>MEASRRDFISIGIGALGAVGGLGALYALVRVMLEPSEIAALGAKTEIDVSKIQPMQVRVTSWKGKTLFAIRLPKDFKPEGYTLKKGALNSKGTTNYEILKGHDVFALVGVCTHLGCIPLWKPQGEGGINKPVFHCPCHGGLYTPYGDVIGGPPPRPLFIPPQKLEGNKLIVGVEGFVKELI[2x];>MGLIEKIVDWIDERAHVREIYRTQMVEYKVAKNLTFPYVFGILALVTFAIQIISGMVLILYYKPSIADAFDSATYSIMGEIPFGWLFRHIHATGANFFMAIVYLHMFTGIYYNAYKRPRELVWIVGWLIYFVLILTALSGYLLPWGQLSYWGFIVTTEIPGSLADAPILKPIFKAIAETIVLWMKGGYVVTDVTLGRVFGSHVLIYPLILLALVGIHLYLVRAAGISNPEGIEYDKKKNPDKFVPFHPYMTLKEGAYVMWYLAVFFFFVFFHISHFLPPENFEPANPLKTPAHIAPEWYLLGYYEVFRSIPSKFWGFVAFNALLLLLLLLPFLDFSPLKSARRRPLFFVMFVIFMISSMALTILGTMPPTPQNAKLGLIFAALVFAFFISLPIISFIEYGWYKAKGGQQE[2x];>MNTWGLIKTIFFAGSTLVFFFLLWFYNPFKHVEHYEVDEEVKAIIDNPWKKTESGKTIAEEGRELFIASCSSCHSLRYDGIYIMSVAANPKWKNIEKTSGRPVYRFGTLYKDRFFVPKDVYEAFAHDDIQGLKASLGQVPPDLSSMYLARGEGYLYQFILNPQKVLPGTTMPQLFNPQFDPQAKEKVAKIVAYMKSVNTPPPKESAKRTVMGVIVIAYFIVMGLLLWKYRENLLKRLGYH[2x]

Cellular respiration complexes convert redox energy into a transmembrane electrochemical proton gradient, which is used to synthesize adenosine triphosphate (ATP) or to transport various substances. In summary, we solved the 3.3 Å structure of respiratory complex III from the hyperthermophilic chemoautotrophic ϵ‐proteobacterium Aquifex aeolicus and revealed the structural basis for the hyperstability of proteins in an extreme thermal environment. The two cyt. b protomers bind to each other mainly through TMH1 and TMH4 to form a stable dimer. Several residues unique for thermophilic bacteria were detected that provide additional stabilization for ligand binding and for the structure of the whole complex.

We also determined the cryo‐EM structure of the cytochrome bc1 complex from A. aeolicus with the Qi site inhibitor antimycin A (AMY). The entire structure of the inhibited enzyme complex is identical with the native structure, except for the Qi site. H, but in the structure with the inhibitor, it is replaced by AMY, suggesting that this inhibitor competitively occupies the Qi site and prevents the entry of the substrate NQ, thus blocking the electron transport and the entire respiratory chain reactions. H.3a In addition, the entire antimycin A inhibitor was found in the Qi pocket and shows a strong interaction with Glu254. There are five hydrogen bonds seen between antimycin A and cyt. b. In contrast, previously only the head group of this inhibitor was reported to be bound to the Qi site.1d, 2c, 16 It is possible that this location represents the NQ channel from the Q‐pool, in which the substrates are transferred into or out of the catalytic center.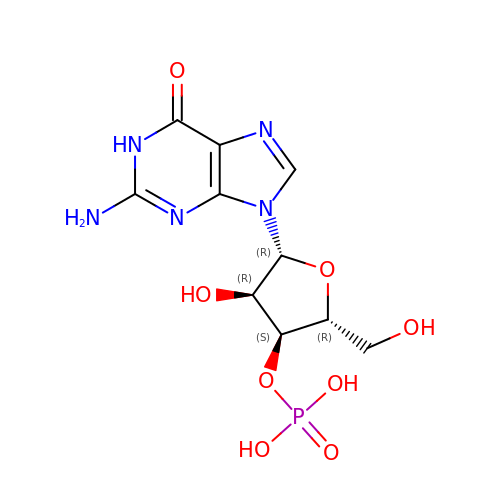GUANOSINE-3'-MONOPHOSPHATE | C10 H14 N5 O8 P | ZDPUTNZENXVHJC-UUOKFMHZSA-N> 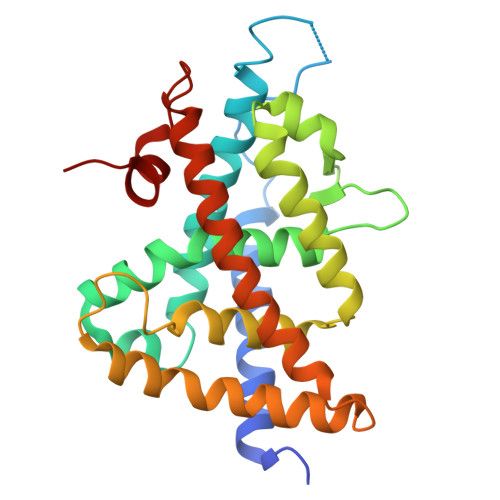GSEGEGVQLTAAQELMIQQLVAAQLQCNKRSFSDQPKVTPWPLGADPQSRDARQQRFAHFTELAIISVQEIVDFAKQVPGFLQLGREDQIALLKASTIEIMLLETARRYNHETECITFLKDFTYSKDDFHRAGLQVEFINPIFEFSRAMRRLGLDDAEYALLIAINIFSADRPNVQEPGRVEALQQPYVEALLSYTRIKRPQDQLRFPRMLMKLVSLRTLSSVHSEQVFALRLQDKKLPPLLSEIWDVHE>[2x]MHHHHHHHHHHSGDEVDAGSGQVDAGTMGTQKVTPALIFAITVATIGSFQFGYNTGVINAPEKIIKEFITKTLTDKGNAPPSEVLLTSLWSLSVAIFSVGGMIGSFSVGLFVNRFGRRNSMLIVNLLAVTGGC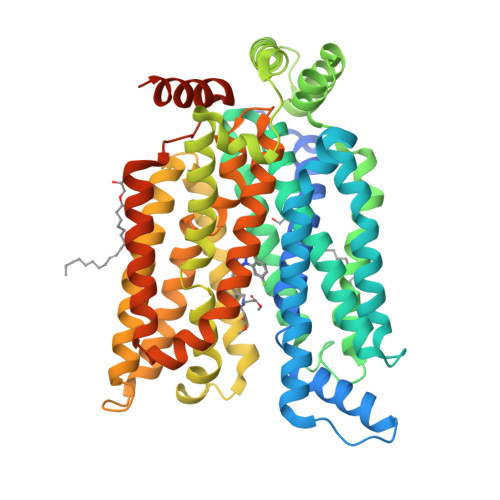FMGLCKVAKSVEMLILGRLVIGLFCGLCTGFVPMYIGEISPTALRGAFGTLNQLGIVVGILVAQIFGLEFILGSEELWPLLLGFTILPAILQSAALPFCPESPRFLLINRKEEENAKQILQRLWGTQDVSQDIQEMKDESARMSQEKQVTVLELFRVSSYRQPIIISIVLQLSQQLSGINAVFYYSTGIFKDAGVQEPIYATIGAGVVNTIFTVVSLFLVERAGRRTLHMIGLGGMAFCSTLMTVSLLLKDNYNGMSFVCIGAILVFVAFFEIGPGPIPWFIVAELFSQGPRPAAMAVAGCSNWTSNFLVGLLFPSAAHYLGAYVFIIFTGFLITFLAFTFFKVPETRGRTFEDITRAFEGQAHGADRSGKDGVMEMNSIEPAKETTTNV>SNAMPKTLTEKLNAIKAAGKGIFVPYIMAGDHEKGLDGLAETIHFLEDLGVSAIEVGIPFSDPVADGPVIEEAGLRSLAHGTSTQALVETLKTIETEIPLVIMTYFNPLFQYGVENFVKDLADTAVKGLIIPDLPHEHANFVEPFLANTDIALIPLVSLTTGIERQKELIEGAEGFIYAVAINGVTGKSGNYRADLDKHLAQLHQVADIPVLTGF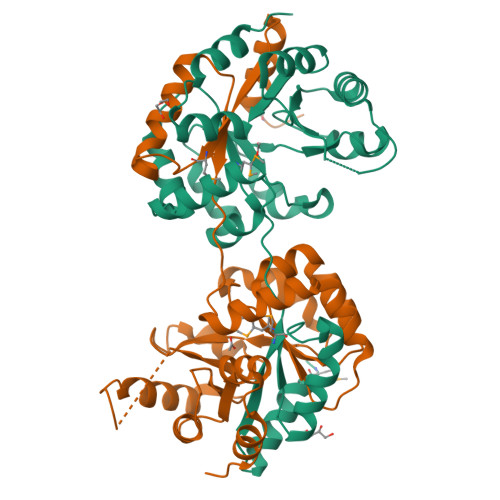GVSSQADLERFNAVSDGVIVGSKIVKALHQGEPIQDFIRQAVAYQK[10x]> ELVRRKSATDIGGLPGKLADCRSTDPRKSELYVVEGDSAGGSAKSGRDSMFQAILPLRGKIINVEKARIDRVLKNTEVQAIITALGTGIHDEFDIGKLRYHKIV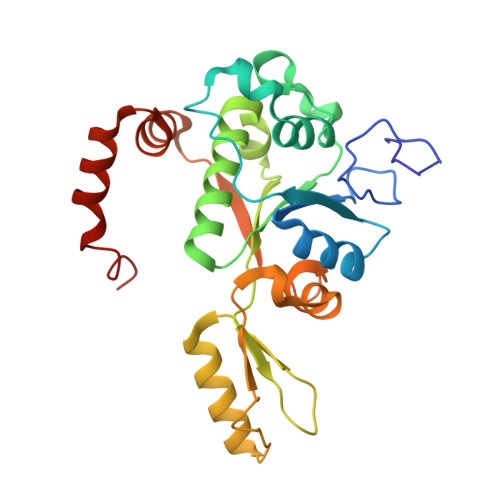LMADADVDGQHISTLLLTLLFRFMRPLIENGHVFLAQPPLYKLKWQRSDPEFAYSDRERDGLLEAGLKAGKKINKEDGIQRYKGLGEMDAKELWETTMDPSVRVLRQVTLDDAAAADELFSILMGEDVDARRSFITRNAKDVRFLDV N-[3-(7H-pyrrolo[2,3-d]pyrimidin-4-yl)phenyl]propanamide 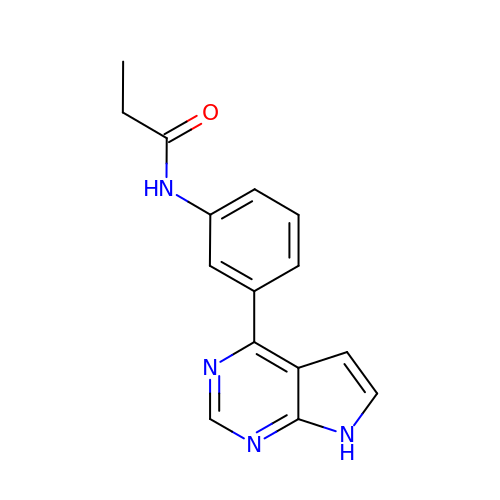| C15 H14 N4 O | KBXLCIHWXYBYSJ-UHFFFAOYSA-N>[2x]SASVRIREAKEGDCGDILRLIRELAEFEKLSDQVKISEEALR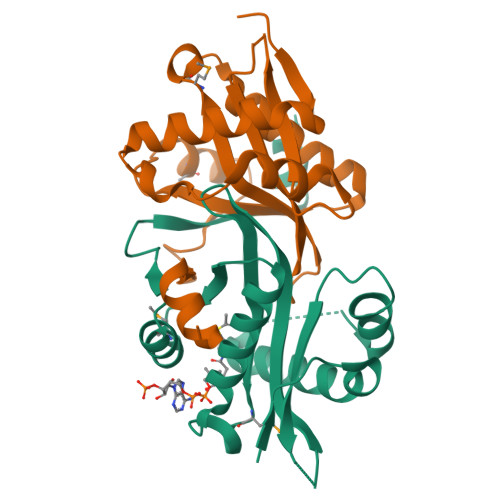ADGFGDNPFYHCLVAEILPAPGKLLGPCVVGYGIYYFIYSTWKGRTIYLEDIYVMPEYRGQGIGSKIIKKVAEVALDKGCSQFRLAVLDWNQRAMDLYKALGAQDLTEAEGWHFFCFQGEATRKLAGK> ASNLKIVRMDRTAGCVTGGEEIM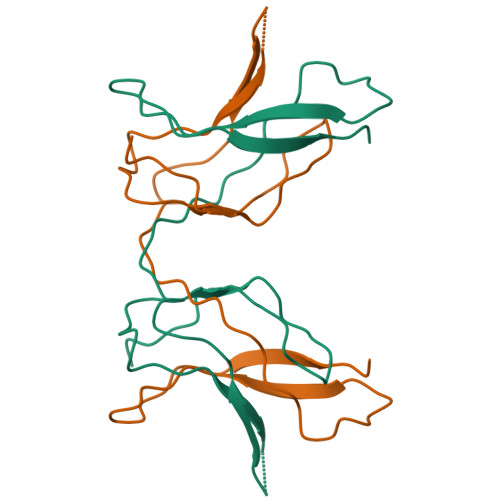LLCDKVQKDDIQIRFYEEEENGGVWEGFGDFSPTDVHRQFAIMFKTPKYKDVNITKPASVFVQLRRKSDLETSEPKPFLYYPE>MTNIFTPIEEALEAYKNGEFLIVMDDEDRENEGDLIMAAELITQEKMAFLVRYSSGYVCVPLSEERANQLELPPMLANRSDRHGTAYTITCDFAEGTTTGISAHDRALTTRSLANPNSKPQDFIKPGHILPLRAVPGLLKKRRGHTEAAVQLSTLAGLQPAGVICELVRDEDGLMMR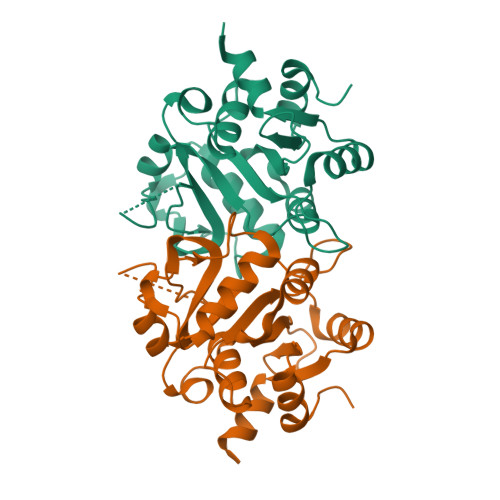LDDCIQFGKKHGIKIININQLVEYISK[2x]> CACACCGT;> TCTGTG;> ACGGACAGCAGTGCA;> GATGCACTGCTG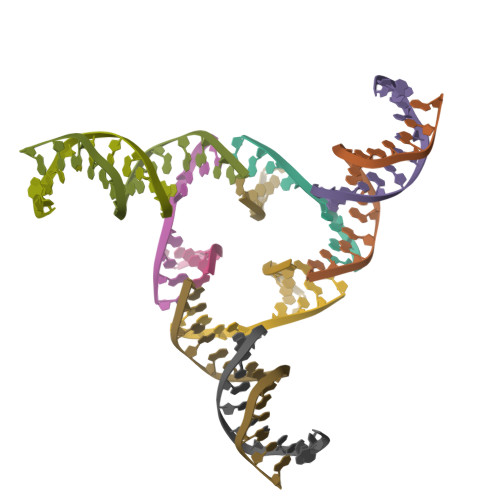T>[2x]XSLSAKDKANVKAIWGKILPKSDEIGEQALSRMLVVYPQTKAYFSHWASVAPGSAPVKKHGITIMNQIDDCVGHMDDLFGFLTKLSELHATKLRVDPTNFKILAHNLIVVIAAYFPAEFTPEIHLSVDKFLQQLALALAEKYR;>VDWTDAERSAIVGLWGKISVDEIGPQALARLLIVSPWTQRHFSTFGNLSTPAAIMGNPAVAKHGKTVMHGLDRAVQNLDDIKNTYVTLSVMHSE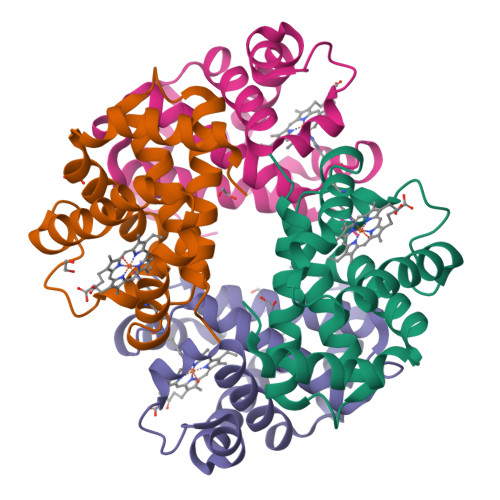KLFVDPDNFRLLADCITVCVAAKLGPAVFSADTQEAFQKFLAVVVSALGRQYH[2x]>[2x]MRILAIDTATEACSVALWNNGTINAHFELCPREHTQRILPMVQEILAASGASLNEIDALAF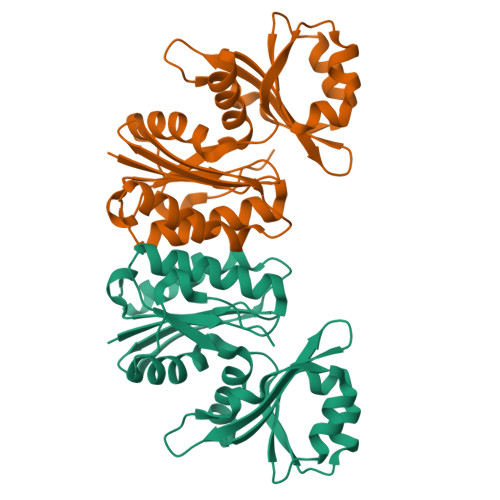GRGPGSFTGVRIGIGIAQGLALGANLPMIGVSTLATMAQGAWRKTGATRVLAAIDARMGEVYWAEYQRDAQGVWQGEETEAVLKPERVGERLKQLSGEWATVGTGWSAWPDLAKECGLTLHDGEVSLPAAEDMLPIASQKLAAGETVAVEHAEPVYLRNEVAWKKLPGKE> QPIFLNVLEAIEPGVVCAGHDNNQPDSFAALLSSLNELGERQLVHVVKWAKALPGFRNLHVDDQMAVIQYSLMGLMVFAMGWRSFTNVNSAMLYFAPDLVFNEYRMHKSRMYSQCVRMRHLSQEFGWLQITPQEFLCMKALLLFSIIPVDGLKNQKFFDELRMNYIKELD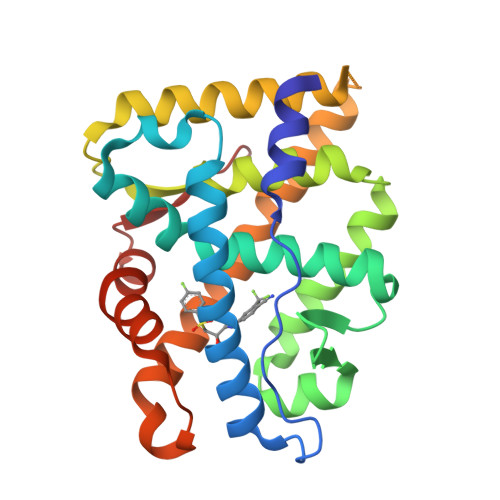RIIACKRKNPTSCSRRFYQLTKLLDSVQPIARELHQFTFDLLIKSHMVSVDFPEMMAEIISVQVPKILSGKVKPIYFHTQ> MHKR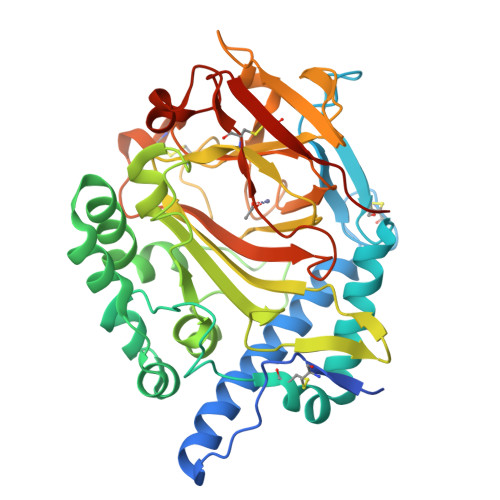FLGTIFGATLTCFQAQAAQFQCQDDVKPTSYTTEEQKLVDQFWNESLIYLDQYLKALETPTGQCKDSAQATIQTYNSETGKMQTQCIMKYRDVELVAKHLKAVLAEPDKAKACFDPQKNYKAFPLYTPSAHVQNLSATSKWINRPLLTDYYKKIGGEIGAAGLELNENFLEITSRTDTTLHWTKDVSIKGLPTLWSSVGWIPFYAENPNAGSDRFRGGYLYAEVMGPWGNLRIKEIDGEKVGAEIGMTAQLFNTSYPYHYHHPQEIYMTLTKPQCIDQNKHMVMHWDNNQFKQKRSDNGWTVNIDGSKGKWKKWFSNQDPEQNWLTYFERNAIHAFHTLEGCNQTIKNSGLVTVWARTTAQDNNQTTQLCRPMTGAKDIKTMKPEDKAICDLDDWKPHHHHHH>GSPNYDKWEMERTDITMKHKLGGGQYGEVYEGVWKKYSLTVAVKTLKEDTMEVEEFLKEAAVMKEIKHPNLVQLLGVCTREPPFYIIIEFMTYGNLLDYLRECNRQEVSAVVLLYMATQISSAMEYLEKKNFIHRDLAARNCLVGENHLVKVADFGLSRLMTGDTYTAHAGAKFPIKWTAPESLAYNKFSIKSDVWAFGVLLWEIATYGMSPYPGIDLSQVYELLEKDYRMERPEGCPEKV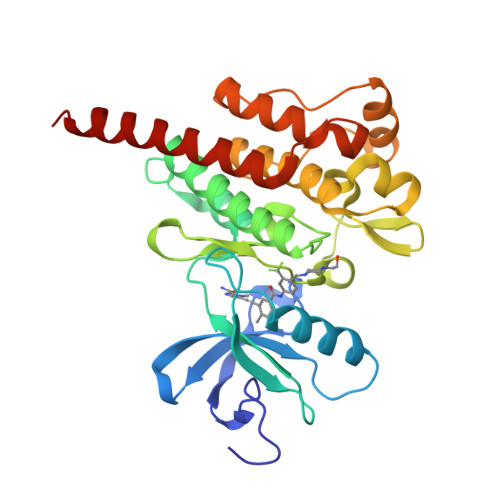YELMRACWQWNPSDRPSFAEIHQAFETMFQESSISDEVEKELG[2x]> MSPRRSAAEAQ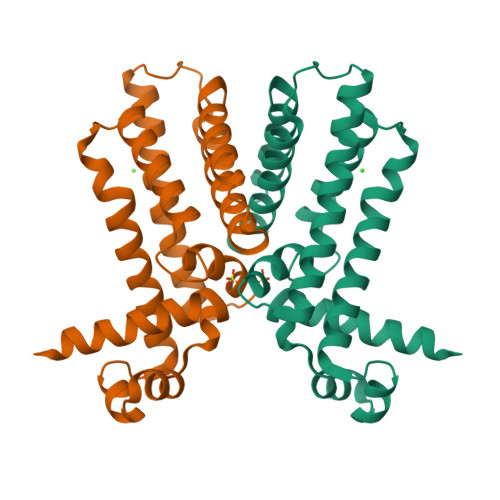ATRGRILGRAAEIASEEGLDGITIGRLAEELEMSKSGVHKHFGTKETLQISTLDKAFVDFWHRVVEPALAEPPGLRRLRAVCANSVGYLEEPLLPGGCLLTAALSEYDGRPGRVRDAVAEVWSRWREQLRADLTAAVDKGELPAGFDVEQALFEIVAAGLALNAAMQLQHDRTAADRARRAIERALAQS> GPGSEVDWNFHKDSFFCDVPSDRYSRVVFTSSGGETLWNLPAIKSMCNVDNSRIRSHPQFGDLCQRTTAASCCPSWTLGNYIAILNNRSSCQKIVERDVSHTLKLLRTCAKHYQNGTLGPDCWDMAARRKDQLKCTNVPRKCTKYNAVYQILHYLVDKDFMTPKTADYATPALKYSMLFSPTEKGESMMNIYLDNFENWNSSDGVTTITGIEFGIKHSLFQDYLLMDTVYPAIAIVIVLLVMCVYTKSMFITLMTMFAIISSLIVSYFLYRVVFHFEFFPFMNLTALIILVGIGANNAFVLCDVWNYTKFDKPHAETSETVSITLQHAALSMFVTSFTTAAAFYANYVSNITAIRCFGVYAGTAILVNYVLMVTWLPAVVVLHERYLLNIFTCFKKPQQQIYDNKSCWTVACQKCHKVLFAISEASRIFFEKVLPCIVIKFRYLWLFWFLALTVGGAYIVCINPKMKLPSLELSEFQVFRSSHPFERYDAEYKKLFMFERVHHGEELHMPITVIWGVSPEDNGNPLNPKSKGKLTLDSSFNIASPASQAWILHFCQKLRNQTFFYQTDEQDFTSCFIETFKQWME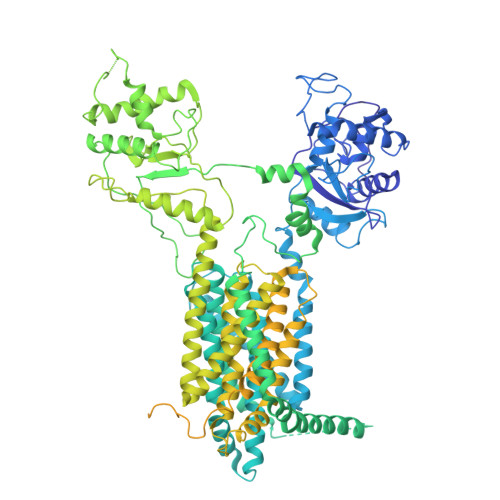NQDCDEPALYPCCSHWSFPYKQEIFELCIKRAIMELERSTGYHLDSKTPGPRFDINDTIRAVVLEFQSTYLFTLAYEKMHQFYKEVDSWISSELSSAPEGLSNGWFVSNLEFYDLQDSLSDGTLIAMGLSVAVAFSVMLLTTWNIIISLYAIISIAGTIFVTVGSLVLLGWELNVLESVTISVAVGLSVNFAVHYGVAYRLAPDPDREGKVIFSLSRVGSAMAMAALTTFVAGAMMMPSTVLAYTQLGTFMMLIMCISWAFATFFFQCMCRCLGPQGTCGQIPLPKKLQCSAFSHALSTSPSDKGQSKTHTINAYHLDPRGPKSELEHEFYELEPLASHSCTAPEKTTYEETHICSEFFNSQAKNLGMPVHAAYNSELSKSTESDAGSALLQPPLEQHTVCHFFSLNQRCSCPDAYKHLNYGPHSCQQMGDCLCHQCSPTTSSFVQIQNGVAPLKATHQAVEGFVHPITHIHHCPCLQGRVKPAGMQNSLPRNFFLHPVQHIQAQEKIGKTNVHSLQRSIEEHLPKMAEPSSFVCRSTGSLLKTCCDPENKQRELCKNRDVSNLESSGGTENKAGGKVELSLSQTDASVNSEHFNQNEPKVLFNHLMGEAGCRSCPNNSQSCGRIVRVKCNSVDCQMPNMEANVPAVLTHSELSGESLLIKTL[(3S)-3-(1H-tetrazol-5-yl)-2,3-dihydro-1H-indol-1-yl][3-(trifluoromethyl)phenyl]methanone | C17 H12 F3 N5 O | 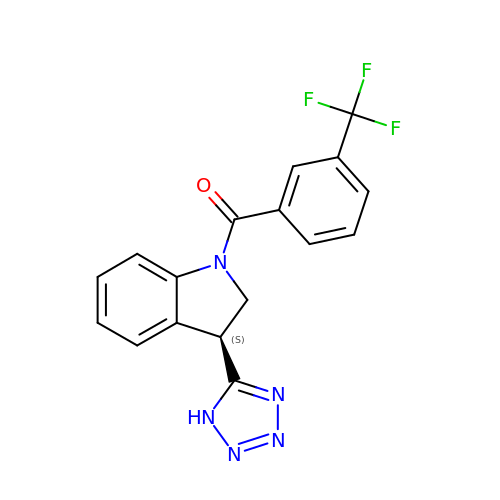ANOXZICGUBIZRA-CYBMUJFWSA-N> MSSGKKPVKVKTPAGKEAELVPEKVWALAPKGRKGVKIGLFKDPETGKYFRHKLPDDYPI

Crenarchaea, one of the two major phyla of cultured archaea, possesses a number of small and basic chromatin proteins, including Sul7d, CC1 and Cren7. In Sulfolobus solfataricus P2, a model strain of Crenarchaeota, Cren7 is synthesized in abundance, constituting ~1% of the total cellular proteins. This protein preferentially binds dsDNA over ssDNA and changes the DNA geometry in vitro. Similar to other Cren7-DNA complexes reported previously, Cren7 binds to the mismatched DNA duplex in the minor groove as a monomer, covering almost all the eight base pairs.

In the crystal of Cren7-GTAATTGC, one protein-DNA complex is found in the asymmetric unit. In crystals, binding of Cren7 to the AT-rich DNA duplex (GTAATTGC) induced opening of T2:G15 but not T10:G7 base pair. Among the most notable structural features of the Cren7-GTAATTGC complex is the flipping of the pyrimidine ring of T2. By contrast, the G15:T2 base pair in this complex appears a totally different conformation with an unusual hydrogen bonding geometry instead of the wobble type. The hydrogen bond from G-O6 to T-N3 has been broken, whereas the G-N1 to T-O2 hydrogen bond (2.75 Å) remains intact. Intriguingly, the hydrogen bond to T-O2 is bifurcated as an additional hydrogen bond is formed from G-N2 to this atom (2.58 Å). Notably, the opening angle of T2:G15 is ~45°, in marked contrast to the slight negative angle of other T:G base pairs. Only three residues on the loop, A29, P30 and K31, are involved in protein-DNA contacts, whereas the hydrogen bonds between the side chain of R33 and the bases of G1 and C16 no longer exist. The distortion of T2:G15 base pair in GTAATTGC leads to the B to A transformation of the G1pT2pA3 steps in addition to the A3pA4 step, while the later is the unique step undergoing this type of transformation in other DNA sequences bound by Cren7. By contrast, the binding affinity of Cren7 for GTAATTGC was 4.6-fold lower than that for the matched DNA.>GAMGSS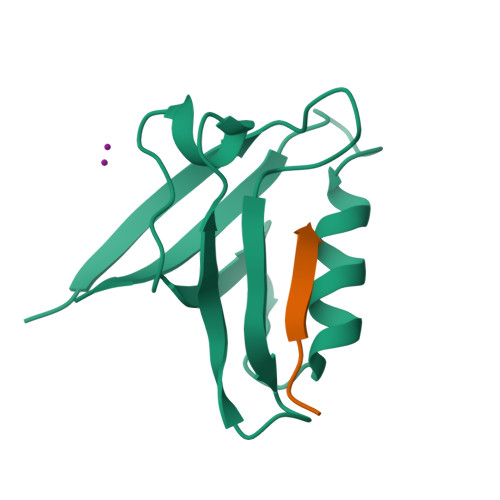TEDASQYYCDKNDNGDSYLVLIRITPDEDGKFGFNLKGGVDQKMPLVVSRINPESPADTCIPKLNEGDQIVLINGRDISEHTHDQVVMFIKASRESHSRELALVIRRR[6x];>[6x]RSSRTRRETQL>[4x]MQGFGVHAMMWSLNWDHESARRAIAGAADYGQDFIEIPLVDLPSVDTAHTRALLEKYGLRAACSLVLPEPAWASVRPEAAVAHLNAALDKAAEMGAEALTGVTYGGTSERTGFPPTQAEYDNLTRALSQSAGHAKTLGLQFGIEAVNRYENHLVNSAEQAVALVERIGADNIFVHLDTFHMNMEEKGIANGIIAAHDYLKYMHMSESDRGTPGFGNVAW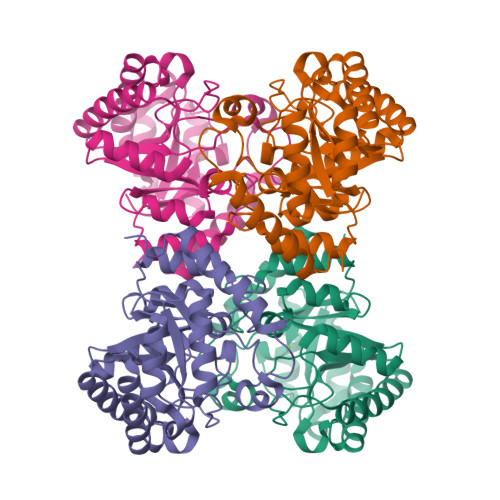DAVFAALAAIGFKGVLTLESFAAMPEEMAGAISTWRPVASGADEVLDKGLAFLRDKASQYRIFGN> RSVYELDCIPLWGVVSIQGNRSEMEDAFAVSPHFLKLPIKMLMGDHEGMSPSLTHLTGHFFGVYDGHGGHKVADYCRDRLHFALAEEIERIKDELC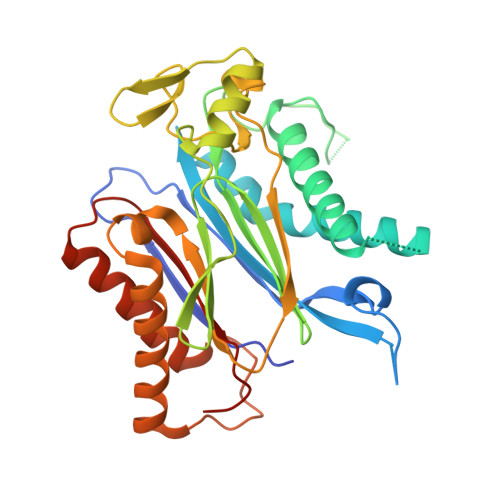KRNTGEGRQVQWDKVFTSCFLTVDGEIEGKIGRAVVGSSDKVLEAVASETVGSTAVVALVCSSHIVVSNCGDSRAVLFRGKEAMPLSVDHKPDREDEYARIENAGGKVIQWQGARVFGVLAMSRSIGDRYLKPYVIPEPEVTFMPRSREDECLILASDGLWDVMNNQEVCEIARRRILMWHKKNGAPPLAERGKGIDPACQAAADYLSMLALQKGSKDNISIIVIDLKAQRKFKTRT> MDREALLQAVKEARELAKPRNFTQSFEFIATLKEIDMRKPENRIKTEVVLPHGRGKEAKIAVIGTGDLAKQAEELGLTVIRKEEIEELGKNKRKLRKIAKAHDFFIAQADLMPLIG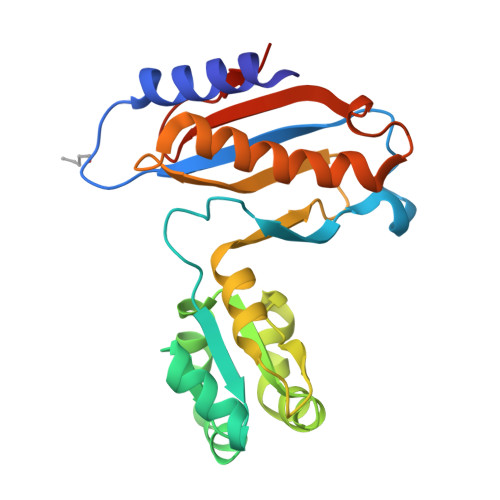RYMGVILGPRGKMPKPVPANANIKPLVERLKKTVVINTRDKPYFQVLVGNEKMTDEQIVDNIEAVLNVVAKKYEKGLYHIKDAYVKLTMGPAVKVKKEKAKKK> TDSFLLRFLRARDFDLDLAWRLLKNY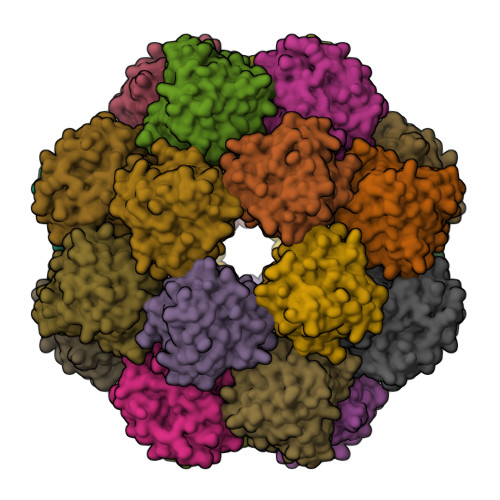YKWRAECPEISADLHPRSIIGLLKAGYHGVLRSRDPTGSKVLIYRIAHWDPKVFTAYDVFRVSLITSELIVQEVETQRNGIKAIFDLEGWQFSHAFQITPSVAKKIAAVLTDSFPLKVRGIHLINEPVIFHAVFSMIKPFLTEKIKERIHMHGNNYKQSLLQHFPDILPLEYGGEEFSMEDICQEWTNFIMKSEDYLSSISE>MHHHHHHSSGRENLYFQGASEALKVVARCRPLSRKEEAAGHEQILTMDVKLGQVTLRNPRAAPGELPKTFTFDAVYDASSKQADLYDETVRPLIDSVLQGFNGTVFAYGQTGTGKTYTMQGTWVEPELRGVIPNAFEHIFTHISRSQNQQYLVRASYLEIYQEEIRDLLSKEPGKRLELKENPETGVYIKDLSSFVTKNVKEIEHVMNLGNQTRAVGSTHMNEVSSRSHAIFIITVECSERGSDGQDHIRVGKLN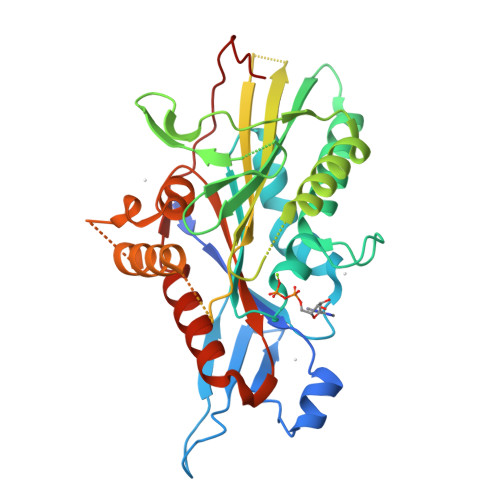LVDLAGSERQNKAGPNTAGGAATPSSGGGGGGGGSGGGAGGERPKEASKINLSLSALGNVIAALAGNRSTHIPYRDSKLTRLLQDSLGGNAKTIMVATLGPASHSYDESLSTLRFANRAKNIKNKPRVNEDPKDTLLREF[2x]>[2x]MHHHHHHITSLYKKAGMAEVPLVYPKENMGESCKAPTLPQPASCPSVPKLPDPFEWSDGSGRVKNLADWECRRNEIKAEIENYELGKKPAPPQSLKATYSGGTLTVVVNDNGGSLTLTSKISVPSGSGPFPVIIGMNSNTGSLSAGQFSDFIQVPFNHDQCAQYSMTGQKNTNAPFYKLYPNLRDA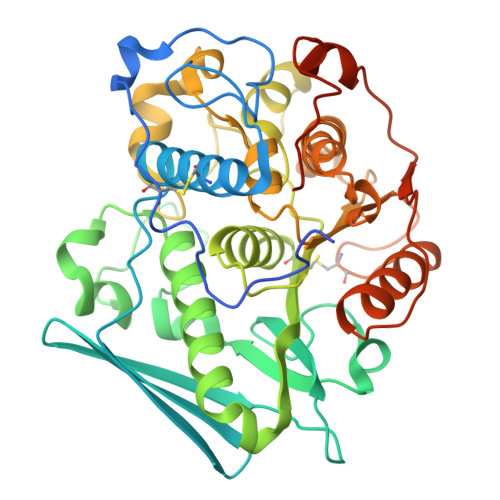GDYIAWSWGISRLIDGIEQVKDQIHADMNHIGVTGCSYAGKMALFGGAFDERVALTIPQESGGGGINAWRVSDTIGNVEKIDNTNYSWFMQALKNNFNGKSDKLPYDHHELIAMVAPRAFFTMGNPDYEWLGDKSGYTSAMAALEVWKAMGVEDRFGFNFVGGHMHCSAAGTQVNDVNKFIDRFLRGKSVSTSNMLSSSVTNDYNSWIAAWKGYTIDTSSTTTTPEDPAFLYKV> EAEPGAAEFAALRNRWVDQITGRNVIQAGDPDFAKAITALNNKAADSLAKLDAAAGRTSVFTDLSLAKDAEMVTTYTRLSQLATAWATPTAAVFGDAAVLAAIKAGLADANTLCYNDRKEEVGNWWSWEIGVPRALADAMVLLHAELSAAERTAYCAAIDHFVPDPWLQFPPKRGKITSVGANRVDLCQGIIIRSLAGEDPTKLNHAVAGLSQVWQYVTSGDGIFRDGSFIQHSTTPYTGSYGVVLLTGLSKLFSLLGGTAFEVSDPTRSIFFDAVEGSFAPVMINGAMADAVRGRSISREANTGYDLGASAIEAILLLARAMDPATAARWRGLCAGWIARDTYRPILNSASVPRTALVKQLEATGVAPVAEATGHKLFPAMDRTMHRGPGWALSLALSSNRIAWYECGNGENNRGYHTGSGMTYFYTSDLGQYDDAFWATANYNRLPGITVDTTPLPDKVEGQWGAAVPADEWSGATALGEVAAVGQHLVGPGRTGLTARKSWFVSGDVTVCLGADISTASGAKVETIVDHRNLHQGSNTLTTAAGTIAGTAGTVEVLGDGRWVHLEGFGGYAMLDDSPLHVLRETRSGSWSGVNINGSATVQQRNFATLYVNHGVGPVAGSYAYMVAPGASVDLTRKLLEGNKYSVIRNDATAQSVEFKTAKTTAATFWKPGMAGDL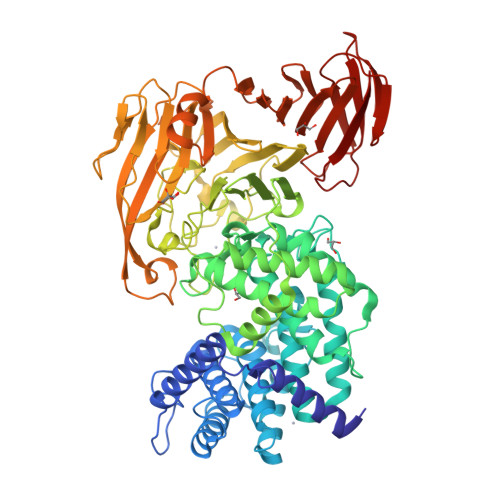GASGPACVVFSRHGNELSLAVSEPTQKAAGLTLTLPEGTWSSVLEGAGTLGTDADGRSTLTLDTTGLSGKTKLIKLKR>[6x]SNAKPRNYQLELALPAMK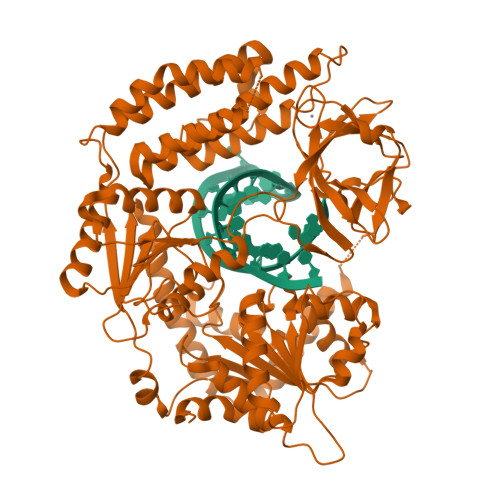GKNTIICAPTGCGKTFVSLLICEHHLKKFPQGQKGKVVFFANQIPVYEQQKSVFSKYFERHGYRVTGISGATAENVPVEQIVENNDIIILTPQILVNNLKKGTIPSLSIFTLMIFDECHNTSKQHPYNMIMFNYLDQKLGGSSGPLPQVIGLTASVGVGDAKNTDEALDYICKLCASLDASVIATVKHNLEELEQVVYKPQKFFRKVESRISDKFKYIIAQLMRDTESLAKRICKDLENLSQIQNREFGTQKYEQWIVTVQKACMVFQMPDKDEESRICKALFLYTSHLRKYNDALIISEHARMKDALDYLKDFFSNVRAAGFDEIEQDLTQRFEEKLQELESVSRDPSNENPKLEDLCFILQEEYHLNPETITILFVKTRALVDALKNWIEGNPKLSFLKPGILTGRGKTNQNTGMTLPAQKCILDAFKASGDHNILIATSVADEGIDIAQCNLVILYEYVGNVIKMIQTRGRGRARGSKCFLLTSNAGVIEKEQINMYKEKMMNDSILRLQTWDEAVFREKILHIQTHEKFIRDSQEKPKPVPDKENKKLLCRKCKALACYTADVRVIEECHYTVLGDAFKECFVSRPHPKPKQFSSFEKRAKIFCARQNCSHDWGIHVKYKTFEIPVIKIESFVVEDIATGVQTLYSKWKDFHFEKIPFDPAE Gabija is one of the most prevalent anti-phage defence systems, occurring in more than 15% of all sequenced bacterial and archaeal genomes, but the molecular basis of how Gabija defends cells from viral infection remains poorly understood. Bacterial Gabija defence operons encode the proteins GajA and GajB, which together protect cells against diverse phages. Gabija protein A (GajA) is a DNA endonuclease that tetramerizes to form the core of the anti-phage defence complex. Two sets of Gabija protein B (GajB) dimers dock at opposite sides of the complex and create a 4:4 GajA–GajB assembly (hereafter, GajAB) that is essential for phage resistance in vivo.

To define the structural basis of Gabija anti-phage defence, we co-expressed Bacillus cereus VD045 GajA and GajB and determined a 3.0 Å X-ray crystal structure of the protein complex. The structure of the GajAB complex reveals an intricate 4:4 assembly with a tetrameric core of GajA subunits braced on either end by dimers of GajB. GajA is a class 2 OLD nuclease, with the Toprim domain containing a complete active site composed of DxD after β3T (D432 and D434), an invariant glutamate after β2T (E379) and an invariant glycine between α1T and β1T (G409). The structure of GajB reveals a superfamily 1A DNA helicase domain. Comparisons with UvrD and Rep show that GajB protomers in the GajAB complex exhibit a partial rotation of the 2B domain relative to 2A–1A–1B, consistent with a partially active conformation that is poised to interact with phage DNA. GajA tetramers form through two highly conserved oligomerization interfaces. First, the GajA N-terminal ATPase domain contains an insertion between β7ABC and β8ABC that consists of four α-helices (α1–α4D) that zip up against a partnering GajA protomer to form a hydrophobic interface along the α2D helix. The GajA ATPase domain contains a second oligomerization interface in a loop between β6ABC and α6ABC, in which hydrogen-bond contacts between D135 and R139 interlock two GajA dimers to form the tetrameric core assembly. Major GajA–GajB contacts also occur in the GajB helicase 1B domain, in which GajA R97 in a loop between α4ABC and β5ABC forms hydrogen-bond contacts with Q150 in GajB α7 along with hydrophobic packing interactions centred at GajB V147. Notably, the GajAB structure shows that the GajB helicase 1A subdomain, which includes the DEXQD-box active site, is positioned adjacent to the GajA ATPase domain, suggesting that GajB ATP hydrolysis and DNA-unwinding activity might regulate the activation of the GajA ATPase domain.

> GSGSGSGSGSSKFSNITIKNFRNFEKVNINLDNKNVIFGMNDIGKTNFLYALRFLLDKEIRKFGFNKSDYHKHDTSKKIEIILTLDLSNYEKDEDTKKLISVVKGARTSANADVFYIALESKYDDKELYGNIILKWGSELDNLIDIPGRGNINALDNVFKVIYINPLVDLDKLFAQNKKYIFEESQGNESDEGILNNIKSLTDQVNQQIGEMTIIKGFQQEITSEYRSLKKEEVSIELKSEMAIKGFFSDIIPYIKKDGDSNYYPTSGDGRRKMLSYSIYNYLAKKKYEDKIVIYLIEEPEISLHRSMQIALSKQLFEQSTYKYFFLSTHSPELLYEMDNTRLIRVHSTEKVVCSSHMYNVEEAYGSVKKKLNKALSSALFAERVLLIEGPSEKILFEKVLDEVEPEYELNGGFLLEVGGTYFNHYVCTLNDLGITHIIKTDNDLKSKKGKKGVYELLGLNRCLNLLGRENLDEITIDIPEDIKGKKKKERLNERKKEIFKQYKNEVGEFLGERIYLSEIDLENDLYSAIGESMKRIFENEDPVHYLQKSKLFNMVELVNNLSTKDCFDVFEHEKFACLKELVGSDRG;> SREQIIKDGGNILVTAGAGSGKTTILVSKIEADLKENKTHYSIAAVTFTNKAAKEIEGRLGYSSRGNFIGTNDGFVESEIIRPFIKDAFGNDYPDNFTAEYFDNQFASYDKGLQVLKYQNILGTYSNPKKNFKFQLALDILKKSLVARQYIFSKYFKIFIDEYQDSDKDMHNLFMYLKDQLKIKLFIVGDPKQSIYIWRGAEPENFNGLIENSTDFNKYHLTSNFRCCQDIQNYSNLFNEETRSLIKEKNEVQNVISIADDMPISDILLKLTEEKQVLNIEAELVILVRRRNQAIEIMKELNEEGFNFIFIPQTPLDRATPNATLLKEVIKYVKNDRYSIYDLAAEIVGNLSSREIKEIQKIINELLVPNINQVLINQVLINLFAKLEITLDTREITAFTEVMMTNEFDIAFDTNEYLHKIFTVHSAKGLEFNQVIITASDYNVHYNRDTNEHYVATTRAKDKLIVIMDNKKYSDYIETLMKELKIKNIIKSI>MDYKDDDDKGTMIEPFGNQYIVARPVYSTNAFEENHKKTGRHHKTFLDHLKVCCSCSPQKAKRIVLSLFPIASWLPAYRLKEWLLSDIVSGISTGIVAVLQGLAFALLVDIPPVYGLYASFFPAIIYLFFGTSRHISVGPFPILSMMVGLAVSGAVSKAVPDRNATTLGLPNNSNNSSLLDDERVRVAAAASVTVLSGIIQLAFGILRIGFVVIYLSESLISGFTTAAAVHVLVSQLKFIFQLTVPSHTDPVSIFKVLYSVFSQIEKTNIADLVTALIVLLVVSIVKEINQRFKDKLPVPIPIEFIMTVIAAGVSYGCDFKNRFKVAVVGDMNPGFQPPITPDVETFQNTVGDCFGIAMVAFAVAFSVASVYSLKYDYPLDGNQELIALGLGNIVCGVFRGFAGSTALSRSAVQESTGGKTQIAGLIGAIIVLIVVLAIGFLLAPLQKSVLAALALGNLKGMLMQFAEIGRLWRKDKYDCLIWIMTFIFTIVLGLGLGLAASVAFQLLTIVFRTQFPKCSTLANIGRTNIYKNKKDYYDMYEPEGVKIFRCPSPIYFANIGFFRRKLIDAVGFSPLRILRKRNKALRKIRKLQKQGLLQVTPKGFICTVDTIKDSDEELDNNQIEVLDQPINTTDLPFHIDWNDDLPLNIEVPKISLHSLILDFSAVSFLDVSSVRGLKSILQEF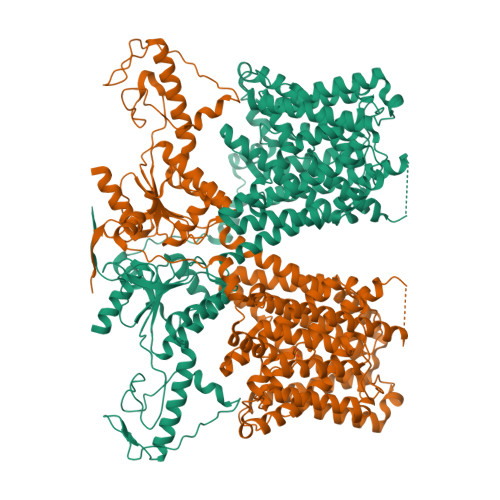IRIKVDVYIVGTDDDFIEKLNRYEFFDGEVKSSIFFLTIHDAVLHILMKKDYSTSKFNPSQEKDGKIDFTINTNGGLRNRVYEVPVETKF[2x]5-cyclopropyl-N-{1-[({trans-4-[(4,4,4-trifluorobutyl)amino]cyclohexyl}methyl)sulfonyl]piperidin-4-yl}-1,2-oxazole-3-carboxamide | C23 H35 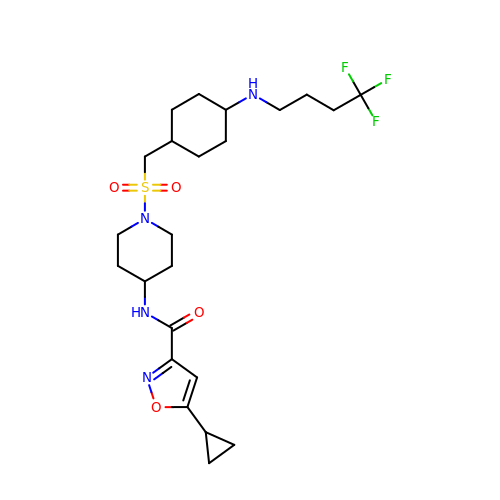F3 N4 O4 S | VAYJCVQRMIULEM-SAABIXHNSA-N[FeFe]-hydrogenases represent one of natures’ most effective classes of redox enzymes catalyzing the reversible reduction of protons to dihydrogen (H2) at turnover frequencies of up to 9000 s-11–3. With their low catalytic over-potential, [FeFe]-hydrogenases represent excellent models for a regenerative and likewise economically feasible H2 production. Their active center (“H-cluster”) can be structured into a standard [4Fe-4S]-cluster ([4Fe]H) and a diiron site ([2Fe]H). Theoretical studies suggest that the most probable PT pathway comprises of strictly conserved residues E282, S319, E279, and C299 (from surface to H-cluster, numbering corresponds to CpI), including two protein-bound water molecules (Wat826, Wat1120 4XDC19, chain B) located between E279 and C29915,16,20. In this study, site-directed mutagenesis (SDM) is used to investigate the PT pathway of two [FeFe]-hydrogenases, namely CpI and HydA1, which represent the largest (M3) and smallest (M1) type of monomeric [FeFe]-hydrogenases, respectively.

Corresponding to earlier crystal structure data, for all CpI variants a space group of P1 21 1 was observed with two copies in the asymmetric unit cell (chain A and B). In wild-type enzyme S319CpI acts as H-bond donor to E282CpI and drags its carboxy group further into the PT pathway. In variant S319ACpI, the carboxyl group of E282CpI is slightly shifted outward, probably due to the lack of the hydroxyl group at position 319CpI. In S319ACpI an unprecedented water molecule (Wat735) is located between E282 and A319, and the nearby water molecule Wat873 of wild-type CpI (chain B) is missing here, suggesting a translocation enabled by the unoccupied space of the missing hydroxyl group of position 319 and the slight outward shift of E282. Although the distance to the carboxyl group of E279 amounts to 5.8 Å, the presence of Wat735 may explain the dramatically diminished yet still detectable H2 release activity of variant S319ACpI (6%).

>MKTIIINGVQFNTDEDTTILKFARDNNIDISALCFLNNCNNDINKCEICTVEVEGTGLVTACDTLIEDGMIINTNSDAVNEKIKSRISQLLDIHEFKCGPCNRRENCEFLKLVIKYKARASKPFLPKDKTEYVDERSKSLTVDRTKCLLCGRCVNACGKNTETYAMKFLNKNGKTIIGAEDEKCFDDTNCLLCGQCIIACPVAALSEKSHMDRVKNALNAPEKHVIVAMAPSVRASIGELFNMGFGVDVTGKIYTALRQLGFDKIFDINFGADMTIMEEATELVQRIENNGPFPMFTSCCPGWVRQAENYYPELLNNLASAKSPQQIFGTASKTYYPSISGLDPKNVFTVTVMPCTSKKFEADRPQMEKDGLRDIDAVITTRELAKMIKDAKIPFAKLEDSEADPAMGEYSGAGAIFGATGGVMEAALRSAKDFAENAELEDIEYKQVRGLNGIKEAEVEINNNKYNVAVINGASNLFKFMKSGMINEKQYHFIEVMACHGGCVNGGGQPHVNPKDLEKVDIKKVRASVLYNQDEHLSKRKSHENTALVKMYQNYFGKPGEGRAHEILHFKYKKSAWSHPQFEK[2x]>MAHHHHHHMAIERTISIIKPDAVGKNVIGKIYSRFEENGLKIVAAKMKQLTLKEAQEFYAVHKDRPFYAGLVEFMTGGPVMIQVLEGENAVLKNRELMGATNPTEAAEGTIRADFATSVSINAVHGS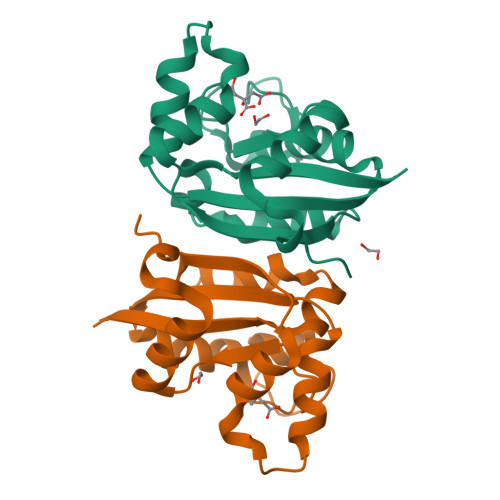DSVENAALEIAYFFSQTEICPR[16x]2-azanylethyl hydrogen sulfate | C2 H7 N O4 S | 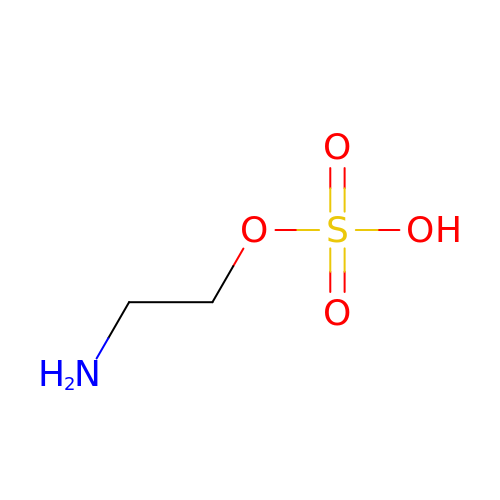WSYUEVRAMDSJKL-UHFFFAOYSA-N> MLEAKFEEASLFKRIIDGFKDCVQLVNFQCKEDGIIAQAVDDSRVLLVSLEIGVEAFQEYRCDHPVTLGMDLTSLSKILRCGNNTDTLTLIADNTPDSIILLFEDTKKDRIAEYSLKLMDIDADFLKIEELQYDSTLSLPSSEFSKIVRDLSQLSDSINIMITKETIKFVADGDIGSGSVIIKPFVDMEHPETSIKLEMDQPVDLTFGAKYLLDIIKGSSLSDRVGIRLSSEAP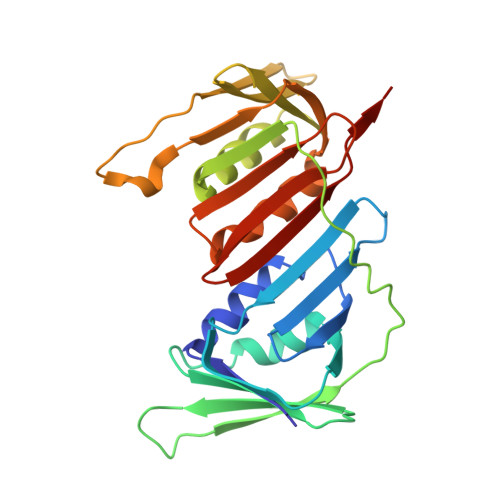ALFQFDLKSGFLQFFLAPKFNDEE>[6x]MVPDRREQSKAKERLLEREEALAKHMSEREKRPPPKIDPPPSPKAPEPSKRVLKEKQAPLFVDTAVEGTLPPLSLLDPAEVKQKSYSPESLEAMSRLL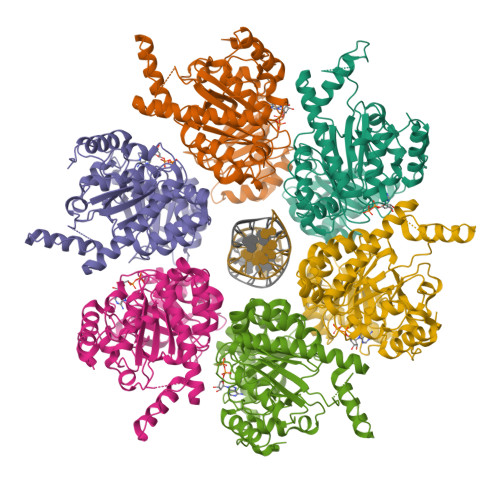EIKLKEFGVEVSVDSVHPGPVITRFEIQPAAGVKVSRISNLAKDLARSLAVISVRVVEVIPGKTTVGIEIPNEDRQMVRFSEVLSSPEYDEHKSTVPLALGHDIGGRPIITDLAKMPHLLVAGTTGSGKSVGVNAMLLSILFKSTPSEARLIMIDPKMLELSIYEGIPHLLCPVVTDMKEAANALRWSVAEMERRYRLMAAMGVRNLAGFNRKVKDAEEAGTPLTDPLFRRESPDDEPPQLSTLPTIVVVVDEFADMMMIVGKKVEELIARIAQKARAAGIHLILATQRPSVDVITGLIKANIPTRIAFQVSSKIDSRTILDQGGAEQLLGHGDMLYLPPGTGLPIRVHGAFVSDDEVHRVVEAWKLRGAPDYIEDILAGVDEGGKLHHHHHH> GTLTGERPPVFWLQGQGCTGCSVTLLNSVHPSIADVLLKVISLEFHPTVMAWEGEHAIEHMRKVAEKFKGKFFLVIEGSVPVEADGK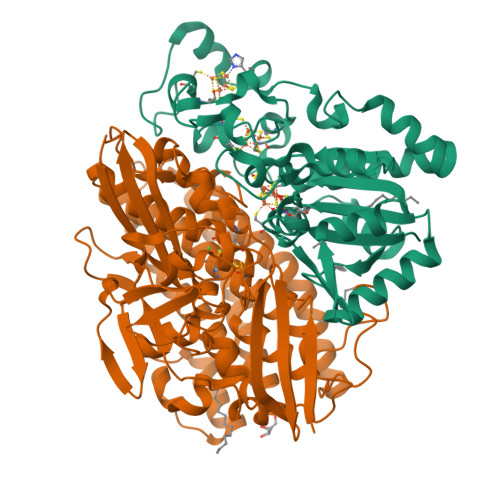YCIIGEANHHEISMVDALKEFGPNAAAVLAVGTCAAYGGIPAAEGSETGATAVSKFLGDNGIKTPVVNIPGCPPHPDWIVGTVVLALDAIKKNGLEGGLAEVVKVLDSDGRPTPFFGRNIHENCPYLDKYDEGVMSATFTDKVGCRYDLGCKGPMTMADCFERKWNGGVNWCVQNAVCIGCVEPDFPDGKSPFYQA;> GATGRTTIAIDPVTRIEGHLKAEVVVENGKVVDARLSGGMYRGFETILRGRDPRDASQIVQRICGVCPTAHSTASVLALDEAFGAKVPNNGRITRNLIFGANYLQSHILHFYHLSAQDFVQGPDTAPFVPRFPKSDLRLSKELNKAGVDQYIEALEVRRICHEMVALFGGRMPHVQGQVVGGATEIPTKEKLVEYAARFKKVRDFVEQKYVPVVYTIGSKYKDMFKVGQGFKAALCVGAFPLDNSGKKHLFMPGVYAKGKDMPFDPSKIKEYVKYSWFAEETTGLNYKEGKTIPAPDKAGAYSFVKAPRYDGLSLEVGPLARMWVNNPELSPVGKKLLKDLFGISAKKFRDLGEEAAFSLMGRHVARAEETYYMLGAIEGWLKEIKAGEDTVVMPAVPASAEGTGFTEAPRGSLLHYVKVKDSKIDNYQIVSASLWNCNPRDDMGQRGAVEEALIGIPVDDIQNPVNVARLIRAFDPULGCAVH>KPIEIIGAPFSKGQPRGGVEKGPAALRKAGLVEKLKETEYNVRDHGDLAFVDVPNDSPFQIVKNPRSVGKANEQLAAVVAETQKNGTISVVLGGDHSMAIGSISGHARVHPDLCVIWVDAHTDINTPLTTSSGNLHGQPVAFLLKELKGKFPDVPGFSWVTPCISAKDIVYIGLRDVDPGEHYIIKTLGIKYFSMTEVDKLGIGKVMEETFSYLLGRKKRPIHLSFDVDGLDPVFTPATGTPVVGGLSYREGLYITEEIYKTGLLSGLDIMEVNPTLGKTPEEVTRTVNTAVALTLSCFGTKREGNHKPETDY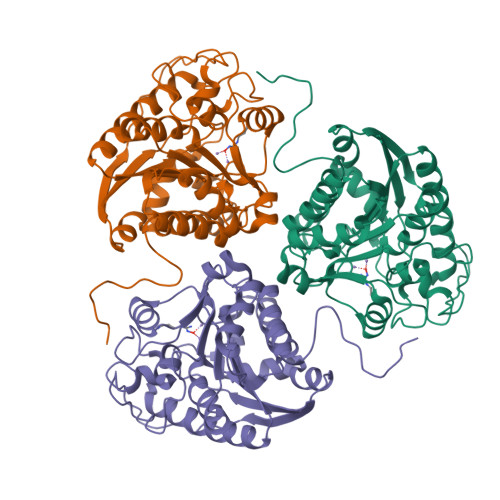L[3x]4-[2-[2-(6-chloranylhexoxy)ethoxy]ethylcarbamoyl]-2-[3-(dimethylamino)-6-(dimethyl-$l^{4}-azanylidene)-10,10-dimethyl-anthracen-9-yl]benzoic acid | C38 H49 Cl N3 O5 | 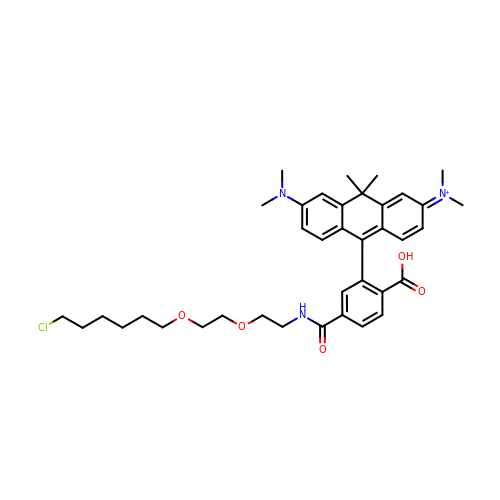BFWDBISDEDTHTG-UHFFFAOYSA-O>[2x]MDETVAEFIKRTILKIPMN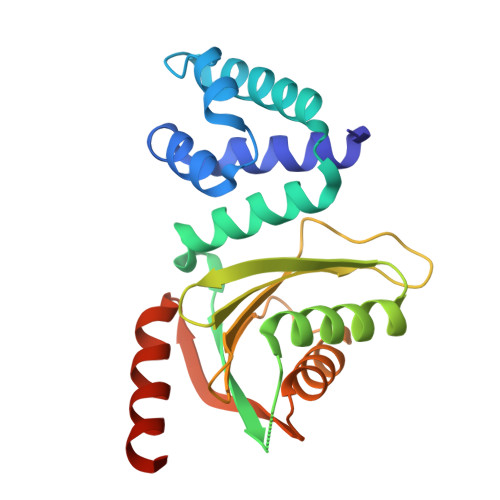ELTTILKAWDFLSENQLQTVNFRQRKESVVQHLIHLCEEKRASISDAALLDIIYMQFHQHQKVWDVFQMSKGPGEDVDLFDMKQFKNSFKKILQRALKNVTVSFRETEENAVWIRIAWGTQYTKPNQYKPTYVVYYSQTPYAFTSSSMLRRNTPLLGQALTIASKHHQIVKMDLRSRYLDSLKAIVFKQYNQTFHHHHHH>[3x]GSPIGIPMSGQSLTDRITAAQHSVTGSAVSKTVCKATTHEIMGPKKKHLDYLIQCTNEMNVNIPQLADSLFERTTNSSWVVVFKSLITTHHLMVYGNERFI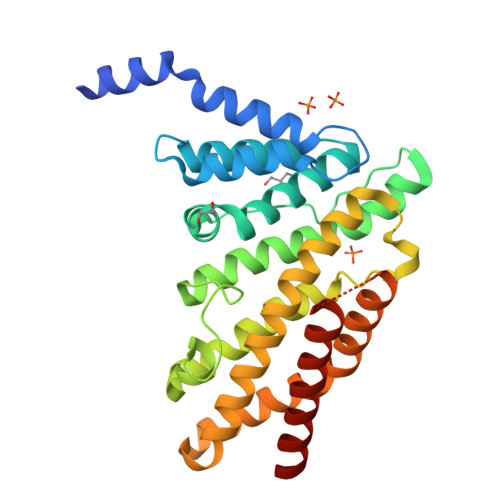QYLASRNTLFNLSNFLDKSGLQGYDMSTFIRRYSRYLNEKAVSYRQVAFDFTKVKRGADGVMRTMNTEKLLKTVPIIQNQMDALLDFNVNSNELTNGVINAAFMLLFKDAIRLFAAYNEGIINLLEKYFDMKKNQCKEGLDIYKKFLTRMTRISEFLKVAEQVGIDRGDISGSGSGHMDRVRNLQSEVEGVKNIMTQNVERILARGENL> MELAEKDKGRDFTLRNARMDDIDQIIKINRLTLPENYPYYFFVEHLKEYGLAFFVAIVDNSVV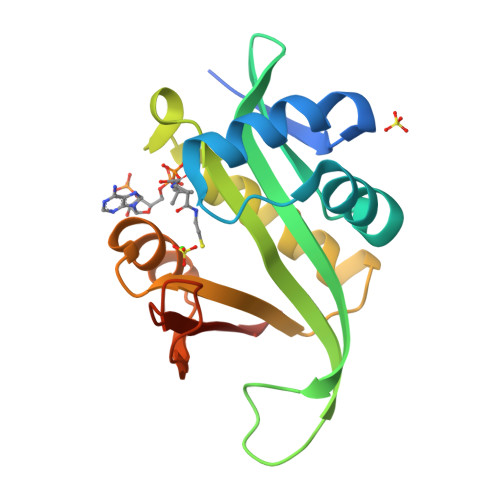GYIMPRIEWGFSNIKQLPSLVRKGHVVSIAVLEEYRRKGIATTLLEASMKSMKNDYNAEEIYLEVRVSNYPAIALYEKLNFKKVKVLKGYYADGEDAYLMARPLHHHHHH> SLSQTTNIKEQTDTGLAPPAP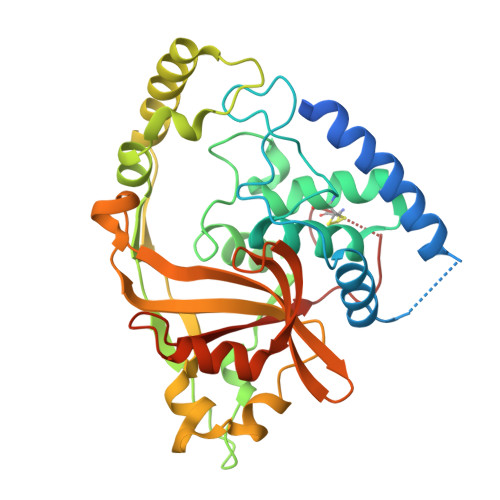AITTNSAAIEEQANSSIRKLYHTLNTMPNTSMADRISQISAYFKGTKYILGSLGEGPNARYDQFPRYRVDGFDCDTYVNTVLSLALANSLESFQECLKHTRYKNGKRSYINRNHFTSIDWNNYNQKRGLLKDITFSIRNEKKQPVALYANALINKPQWYNHKTIDTIRLQKQDKNEQEKRLVELKAKGKTLETSLSNVPYIPFTALFSENKPNLHLFSQIPNGAVIEIIRPNWDLRQQIGTELDISHLGFAIWINNELFFRQASSQYGKVVDVSLIDYLDKARSSPTIKGINIQVVLPEKPVSNGCQLFDIR> MTSLFEPAQAGDIALANRIVMAPLT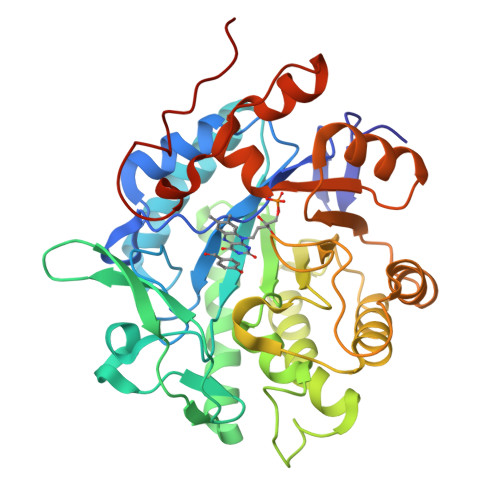RNRSPGAIPNNLNATYYEQRATAGLIVTEGTPISQQGQGYADVPGLYKREAIEGWKKITDGVHSAGGKIVAQIWHVGRISHTSLQPHGGQPVAPSAITAKSKTYIINDDGTGAFAETSEPRALTIDDIGLILEDYRSGARAALEAGFDGVEIHAANGYLIEQFLKSSTNQRTDDYGGSIENRARFLLEVVDAVAEEIGAGRTGIRLSPVTPANDIFEADPQPLYNYVVEQLGKRNLAFIHVVEGATGGPRDFKQGDKPFDYASFKAAYRNAGGKGLWIANNGYDRQSAIEAVESGKVDAVAFGKAFIANPDLVRRLKNDAPLNAPNQPTFYGGGAEGYTDYPALAQHHHHHH4-[(E)-3-(3,5-ditert-butylphenyl)-3-oxidanylidene-prop-1-enyl]benzoic 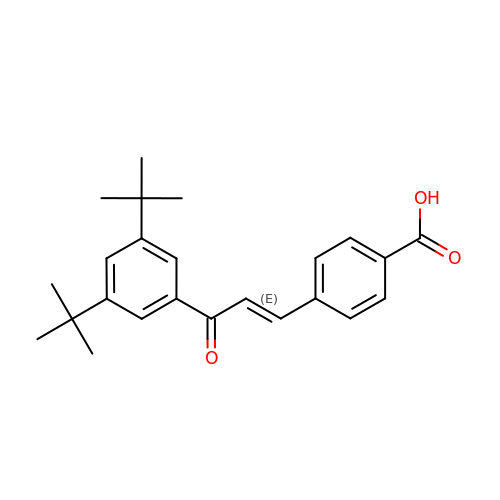acid | C24 H28 O3 | FOUVTBKPJRMLPE-FMIVXFBMSA-N>TQKPHLGNAGDSVTLNDVANVMYYGEAQIGDNKQKFAFIFDTGSANLWVPSAQCNTIGCKTKNLYDSNKSKTYEKDGTKVEMNYVSGTVSGFFSKDIVTIANLSFPYKFIEVTDTNGFEPAYTLGQFDGIVGLGWKDLSIGSVDPVVVELKNQNKIEQAVFTFYLPFDDKHKGYLTIGGIEDRFYEGQLTYEKLNHDLYWQVDLDLHFGNLTVEKATAIVDSGTSSITAPTEFLNKFFEGLDVVKIPFLPLYITTCNNPKLPTLEFRSATNVYTLEPEYYLQQIFDFGISLCMVSIIPVDLN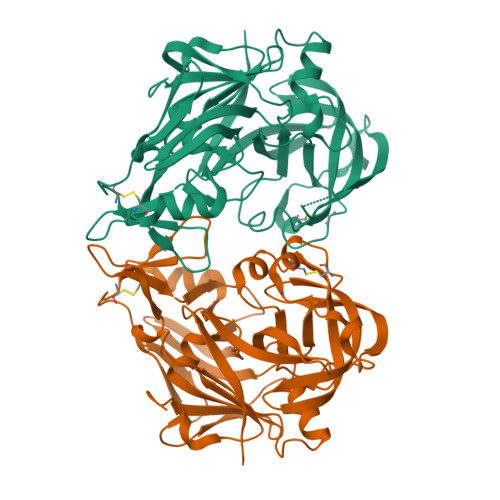KNTFILGDPFMRKYFTVFDYDNHTVGFALAKKKL[2x]>XEKNALLRYLLDKDX[13x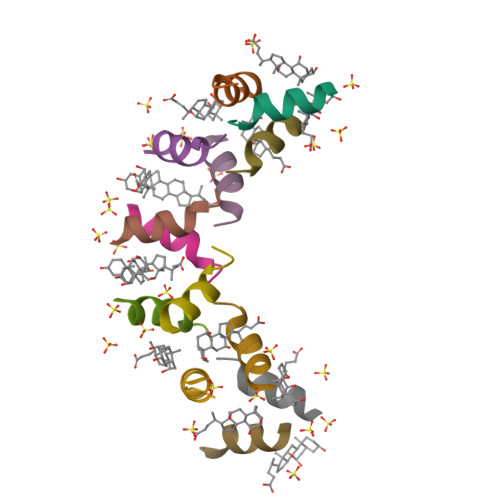]>MSVFSLKIDIADNKFFNGETSPLFSQSQAKLARQFHQKIAGYRPTPLCALDDLANLFGVKKILVKDESKRFGLNAFKMLGGAYAIAQLLCEKYHLDIETLSFEHLKNAIGEKMTFATTTDGNHGRGVAWAAQQLGQNAVIYMPKGSAQERVDAILNLGAECIVTDMNYDDTVRLTMQHAQQHGWEVVQDTAWEGYTKIPTWIMQGYATLADEAVEQMREMGVTPTHVLLQAGVGAMAGGVLGYLVDVYSPQNLHSIIVEPDKADCIYRSGVKGDIVNVGGDMATIMAGLACGEPNPLGWEILRNCAT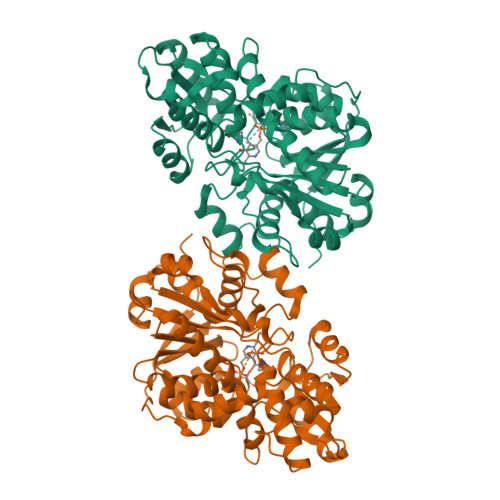QFISCQDSVAALGMRVLGNPYGNDPRIISGESGAVGLGVLAAVHYHPQRQSLMEKLALNKDAVVLVISTEGDTDVKHYREVVWEGKHAVAP[2x]> MHHHHHHMPIIEQVRAREILDSRGNPTVEVEVALIDGTFARAAVPSGASTGEHEAVELRDGGDRYGGKGVQKAVQAVLDEIGPAVIGLNADDQRLVDQALVDLDGTPDKSRLGGNAILGVSLAVAKAAADSAELPLFRYVGGPNAHILPVPMMNILNGGAHADTAVDIQEFMVAPIGAPSFVEALRWGAEVYHALKSVLKKEGLSTGLGDEGGFAPDVAGTTAALDLISRAIESAGLRPGADVALALDAAATEFFTDGTGYVFEGTTRTADQMTEFYAGLLGAYPLVSIEDPLSEDDWDGWAALTASIGDRVQIVGDDIFVTNPERLEEGIERGVANALLVKVNQIGTLTETLDAVTLAHHGGYRTMISHRSGETEDTMIADLAVAIGSGQIKTGAPARSERVAKYNQLLRIEEALGDAARY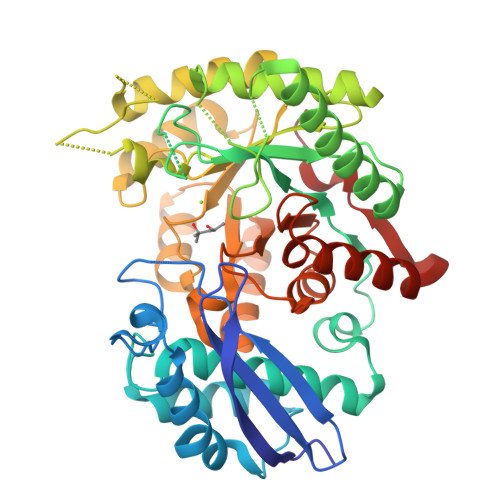AGDLAFPRFACET Amongst the Arabidopsis MSL channels, MSL10 is enigmatic in that it has two separable functional modalities, regulated cell death signaling conferred by its N-terminal soluble ‘death’ domain and force-activated ion channel activity imparted by its C-terminal portion. When heterologously expressed in Xenopus oocytes, MSL10 is indeed activated by membrane stretch and displays a preference for anions. In Arabidopsis, MSL10 is primarily expressed in the shoot apex, root tips, and vascular tissues, playing a critical role in adaptation to hypo-osmotic shock and induction of programmed cell death. Analogous to DmMSL10/FLYC1, each subunit of the heptameric AtMSL10 channel is composed of a transmembrane domain (TMD) with six membrane-spanning helices (TM1-TM6) and a characteristic C-terminal cytoplasmic domain (CTD) shared by all MscS homologs.

In addition to the characteristic TM4-TM5 CLD, we observed an inter-subunit salt bridge between E534 and K539 at the extracellular end of TM5-TM6, which is unique to AtMSL10. We introduced two single-point charge reversal mutations at these two positions, E534K or K539E, to disrupt the inter-subunit salt bridge interaction. Surprisingly, both mutations virtually maintained the wild-type channel activity, as assessed in excised membrane patches from Xenopus oocytes. We determined the cryo-EM structure of K539E at ~3.7 Å resolution, which represents an open conformation nearly identical to that of the wild type (r.m.s.d of ~0.3 Å for all Cα atoms). Interestingly, densities corresponding to the TMD and the TM4-TM5 linker domain are better resolved in the K539E mutant than in the wild type. Thus, the extracellular E534-K539 salt bridge between two adjacent subunits in the heptameric AtMSL10 channel is not required for the non-domain swapped arrangement or channel gating by membrane tension.

>MAEQKSSNGGGGGGDVVINVPVEEASRRSKEMASPESEKGVPFSKSPSPEISKLVGSPNKPPRAPNQNNVGLTQRKSFARSVYSKPKSRFVDPSCPVDTSILEEEVREQLGAGFSFSRASPNNKSNRSVGSPAPVTPSKVVVEKDEDEEIYKKVKLNREMRSKISTLALIESAFFVVILSALVASLTINVLKHHTFWGLEVWKWCVLVMVIFSGMLVTNWFMRLIVFLIETNFLLRRKVLYFVHGLKKSVQVFIWLCLILVAWILLFNHDVKRSPAATKVLKCITRTLISILTGAFFWLVKTLLLKILAANFNVNNFFDRIQDSVFHQYVLQTLSGLPLMEEAERVGREPSTGHLSFATVVKKGTVKEKKVIDMGKVHKMKREKVSAWTMRVLMEAVRTSGLSTISDTLDETAYGEGKEQADREITSEMEALAAAYHVFRNVAQPFFNYIEEEDLLRFMIKEEVDLVFPLFDGAAETGRITRKAFTEWVVKVYTSRRALAHSLNDTKTAVKQLNKLVTAILMVVTVVIWLLLLEVATTEVLLFFSTQLVALAFIIGSTCKNLFESIVFVFVMHPYDVGDRCVVDGVAMLVEEMNLLTTVFLKLNNEKVYYPNAVLATKPISNYFRSPNMGETVEFSISFSTPVSKIAHLKERIAEYLEQNPQHWAPVHSVVVKEIENMNKLKMALYSDHTITFQENRERNLRRTELSLAIKRMLEDLHIDYTLLPQDINLTKKNSLEVLFQ[7x]>DFGTPEMLPHVQCKNSTNSTTLVSWAEPASKHHGYILCYKKTPSEKCENLANDVNSFEVKNLRPYTEYTVSLFAYVIGRVQRNGPAKDCNFRTKAARPGKVNGMKTSRASDNSINVTCNSPYEINGPEARYILEVKSGGSLVKTFNQSTCKFVVDNLYYSTDYEFLVYFYNGEYLGDPEIKPQSTS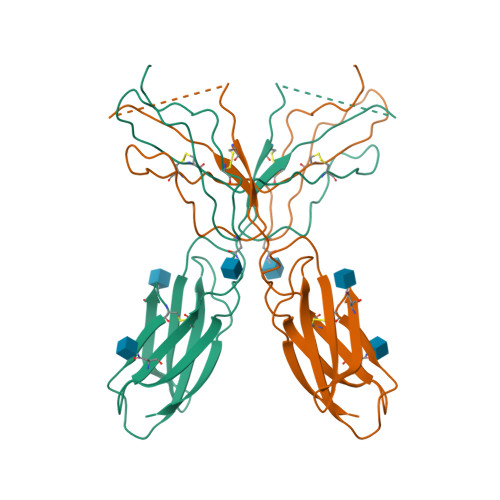YNSK[2x]1-(5-O-phosphono-beta-D-ribofuranosyl)-1H-imidazole 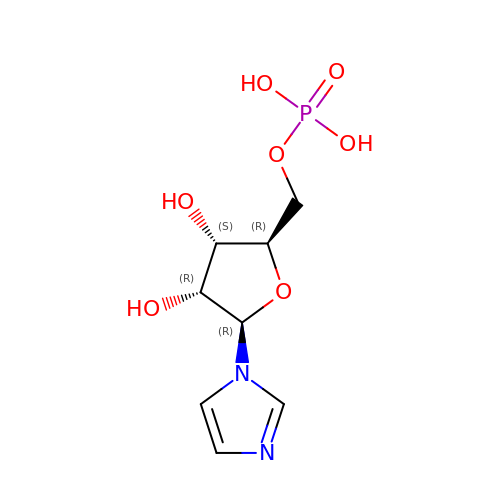| C8 H13 N2 O7 P | YEBULYOZZUNFGU-WCTZXXKLSA-N>MSHQLKIIADGKALSLLAAVDVDTCYRVNSIPSATLKLSVPDRPLSSFSQTDVQTELAHCQVGKTL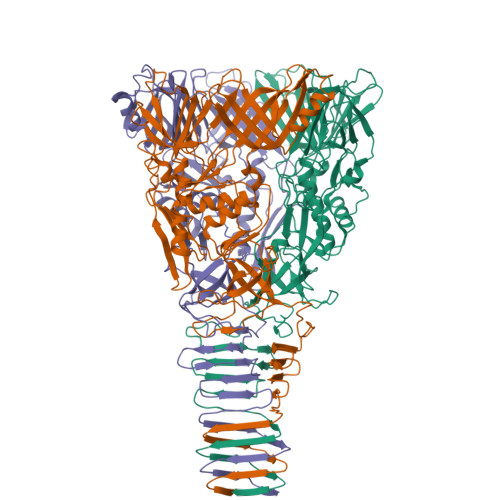RLELIDGSKKWVLFNGLITRKALRIKNKQLLLTLVVKHRLQLMVDTQHSQLFKDKSEKAILSTLLNQTGINARFGKIAALDQKHEQMVQFRCSDWHFLLCRLSATGAWLLPAIEDVQFVQPDALKSNSAYTLKSRGDENKDIVVKDAYWQFDNQINPALLEVSGWDISKQQVQSGGRYGKIALGKAALSPDGLASLNKTGWDICYSSPLTTQESGYLAQGLLLNQRISGVTGEFLLKGDGRYQLGDNIQLTGFGSQLDGTASITEVRHRLNRRIDWETTVSIGLQHEYLPILPDAPELHIATVAKYQQDSAVLNRIPIILPVLNRPNEFLWARLGKPYASHESGFCFYPEPGDEVIIGFFENDPRYPVILGAMHNPKNKAPFEPTQDNREKVLIVKKGEAQQQLVIDGKEKMIRINAGENQIMLQQDKDISLSTKKELTLKAQTMNATMDKSLAMSGKNSVEIKGAKINLTQ[3x]5-[(1E)-2-(2-methoxyphenyl)hex-1-en-1-yl]furo[2,3-d]pyrimidine-2,4-diamine 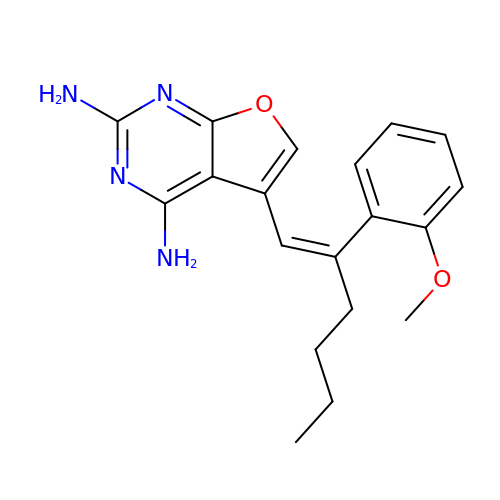| C19 H22 N4 O2 | OJEFVGFDNJBOHB-ZRDIBKRKSA-N>[2x]GSRAYSFKVVLLGEGCVGKTSLVLRYCEN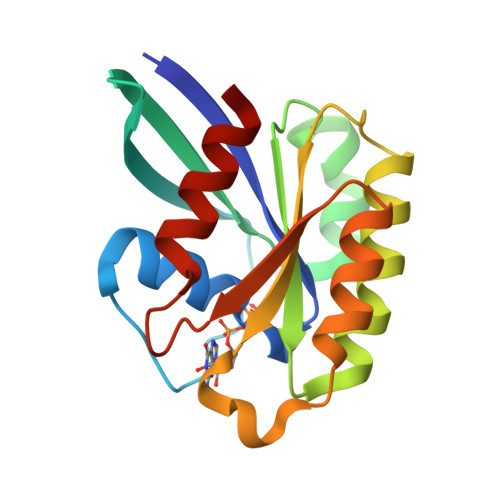KFNDKHITTLQASFLTKKLNIGGKRVNLAIWDTAGQERFHALGPIYYRDSNGAILVYDITDEDSFQKVKNWVKELRKMLGNEICLCIVGNKIDLEKERHVSIQEAESYAESVGAKHYHTSAKQNKGIEELFLDLCKRMIET>MSPGPQSGGQERGSMERKMVELEDTGLTFATEVDLERLQALAAEWLQVIGEDPGREGLLKTPERVAKAWAFLTRGYRQRLEEVVGGAVFPAEGSEMVVVKGVEFYSMCEHHLLPFFGKVHIGYIPDGKILGLSKFARIVDMFARRLQVQERLAVQI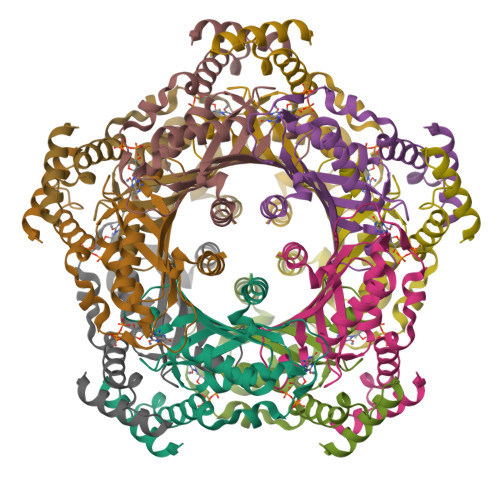AEAIQEVLEPQGVGVVVEGVHLCMMMRGVEKQHSRTVTSAMLGVFRENQKTREEFLSHLRDGTA[5x]>STASRALSQNGNIENPRPSKVQELSVYEINELDRHSPKILKNAFSLMFGLGDLVPFTNKLYTGDLKKRVGITAGLCVVIEHVPEKKGERFEATYSFYFGDYGHLSVQGPYLTYEDSFLAITGGAGIFEGAYGQVKLQQLVYPTKLFYTFYLKGLANDLPLELTGTPVPP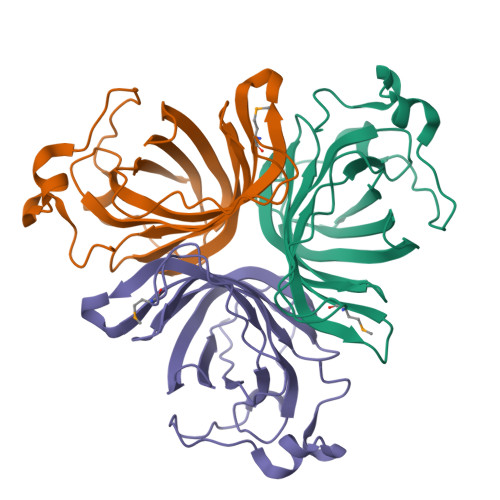SKDIEPAPEAKALEPSGVISNYTN[3x]>[2x]GSHLWQMDNTHWNKTIIWVAVETNSGLVEAQVIPEETALQVALCILQLIQRYTVLHLHSDNGPCFTAHRIENLCKYLGITKTTGIPYNPQSQGVVERAHRDLKDRL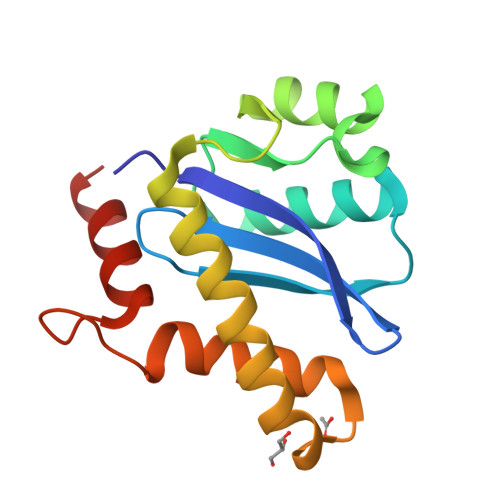AAYQGDCETVEAALSLALVSLNKKRGGIGGHTPYEIYLESEHTKYQ> GAVDLNKENRDPKYVESIVNRSQKIVDKLGLTDAKVAEDVCNVIANRYFELNDIYEIRDAKV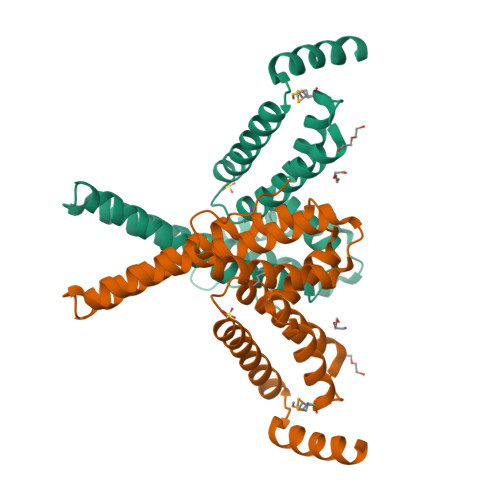KAVKESGLTGDAKNEALKAAENEKDAALYRSHFAFPASLSLFLNEEQIEAVKDGMTYGVVKVTYEATLDMIPSLKEEEKVQIYAWLVEAREFAMDAENSNKKHAAFGKYKGRINNYLAKRGYNLTKEREEWAKRVKARGGTL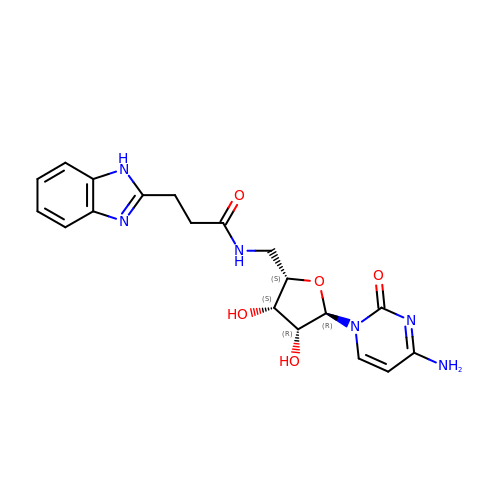4-AMINO-1-(5-{[3-(1H-BENZIMIDAZOL-2-YL)PROPANOYL]AMINO}-5-DEOXY-ALPHA-L-LYXOFURANOSYL)PYRIMIDIN-2(1H)-ONE | C19 H22 N6 O5 | IHRYIMVLMZNCKA-FCRVUTKVSA-N Coronaviruses use an RdRp enzyme to carry out replication and transcription of their RNA genome. The RdRp consists of three non-structural protein (nsp) subunits, the catalytic subunit nsp126 and the accessory subunits nsp8 and nsp73,7. For RNA-dependent RNA elongation, the 3ʹ-terminal nucleotide of the RNA product chain resides in the –1 site and the incoming nucleoside triphosphate (NTP) substrate binds to the adjacent +1 site. Catalytic nucleotide incorporation then triggers RNA translocation and liberates the +1 site for binding of the next incoming nucleoside triphosphate (NTP).

We prepared RNA scaffolds containing RMP at positions –3 or –4 by annealing short RMP-containing oligonuclotides to long, loop-forming RNAs (scaffolds 1 and 2, respectively). The first RdRp-RNA structure (structure 1) was resolved at 3.1 Å resolution and showed that the RMP was located at position –3 of the RNA product strand, as expected from the design of scaffold 1. The RdRp-RNA complex adopted the post-translocated state. The RNA 3ʹ-end resided in the –1 site and the +1 site was free to bind the next NTP substrate. The 1ʹ-cyano group of the RMP ribose moiety was located at position –3 and is accommodated there by an open space in the RNA product-binding site of the RdRp. Thus, structure 1 represents an active state of the elongation complex that is poised to add one more nucleotide to the RNA before stalling, consistent with biochemical results.

> SNASADAQSFLNRVCGVSAARLTPCGTGTSTDVVYRAFDIYNDKVAGFAKFLKTNCCRFQEKDEDDNLIDSYFVVKRHTFSNYQHEETIYNLLKDCPAVAKHDFFKFRIDGDMVPHISRQRLTKYTMADLVYALRHFDEGNCDTLKEILVTYNCCDDDYFNKKDWYDFVENPDILRVYANLGERVRQALLKTVQFCDAMRNAGIVGVLTLDNQDLNGNWYDFGDFIQTTPGSGVPVVDSYYSLLMPILTLTRALTAESHVDTDLTKPYIKWDLLKYDFTEERLKLFDRYFKYWDQTYHPNCVNCLDDRCILHCANFNVLFSTVFPPTSFGPLVRKIFVDGVPFVVSTGYHFRELGVVHNQDVNLHSSRLSFKELLVYAADPAMHAASGNLLLDKRTTCFSVAALTNNVAFQTVKPGNFNKDFYDFAVSKGFFKEGSSVELKHFFFAQDGNAAISDYDYYRYNLPTMCDIRQLLFVVEVVDKYFDCYDGGCINANQVIVNNLDKSAGFPFNKWGKARLYYDSMSYEDQDALFAYTKRNVIPTITQMNLKYAISAKNRARTVAGVSICSTMTNRQFHQKLLKSIAATRGATVVIGTSKFYGGWHNMLKTVYSDVENPHLMGWDYPKCDRAMPNMLRIMASLVLARKHTTCCSLSHRFYRLANECAQVLSEMVMCGGSLYVKPGGTSSGDATTAYANSVFNICQAVTANVNALLSTDGNKIADKYVRNLQHRLYECLYRNRDVDTDFVNEFYAYLRKHFSMMILSDDAVVCFNSTYASQGLVASIKNFKSVLYYQNNVFMSEAKCWTETDLTKGPHEFCSQHTMLVKQGDDYVYLPYPDPSRILGAGCFVDDIVKTDGTLMIERFVSLAIDAYPLTKHPNQEYADVFHLYLQYIRKLHDELTGHMLDMYSVMLTNDNTSRYWEPEFYEAMYTPHTVLQ;> SNAAIASEFSSLPSYAAFATAQEAYEQAVANGDSEVVLKKLKKSLNVAKSEFDRDAAMQRKLEKMADQAMTQMYKQARSEDKRAKVTSAMQTMLFTMLRKLDNDALNNIINNARDGCVPLNIIPLTTAAKLMVVIPDYNTYKNTCDGTTFTYASALWEIQQVVDADSKIVQLSEISMDNSPNLAWPLIVTALRANSAVKLQ;> SNASKMSDVKCTSVVLLSVLQQLRVESSSKLWAQCVQLHNDILLAKDTTEAFEKMVSLLSVLLSMQGAVDINKLCEEMLDNRATLQ> PALSYGGDLDVTQGAQTLQDVLTEAAKTTNGLTYIVNSKNELTQSYAQLQGDAERVLTGLRALGLKAGDPVFFQFSSNHAMVTAFWACVLGGFVPTLVSAAPTYREMNAAVKKLHHAWKLLEHPLILTDDSLIEEVQGLAFLWHTDQLRVAAVEPMLTLERDTAAHPAAPDDSVFFILTSGSTGMPKCVEHSHRSVLANVKGTVAANQFTQEDVSLDWMPLDHIGGIVMFHLVNVYTGCEQIRARTDDFIAQPLRWLDWMDRYRATKTWAPNFAFAMINDYEKEISSGSWDLSAMTCMINGAEAVVPKTIHRFLHLLAPHGLKGDVIRPAFGMSEISSAVVFSFAIERGDENSGVLTFEETSLTEQLRPAEARETGTVSFTELGKPIPGITIRIVNHQHELLPEDHIGRVQIKGPTTMKGYYRNDEANQEVFQADGWFHTGDLGFLHEGRLTLTGREKDMIIINGKNYHNYEIEAIAEEVPGVETSFVAACSVRMEASASDELILFFTPKLYEPAYIMRASQHIKSHIATKMGLSASRIIPVQKHAFPKTSSGKIERAQLKTRW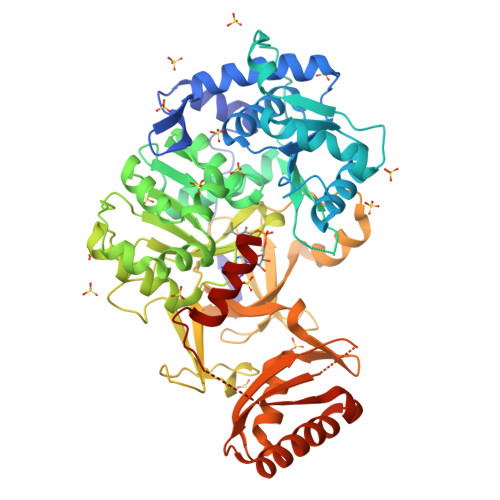QEGAAAENLYFQ>SNAMTQYTHIRNATGKLTIKNTTFLIDPFLAPKDTYPGFEGTFNYQQRMPMVDLPLSMDDLLSNVTAVVVTHTHLDHWDDTAINSIPKSLPIFVQNTADKELITSQGFIDVRIIFESLEFNGITLRKTGGSHGTVEMYANPVL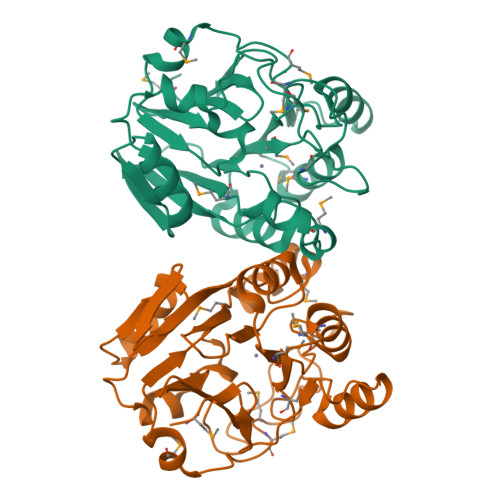APLAGDAMGVIFEAADEPTVYLVGDTVWTSDVEKALLRFDPNVIIMNTGYAQILGFEDSIIMGTKDIGRMVVRKPEAKIIAVHMDTVNHTATSRKDVRKFIKGNNIESHVAVPEDGETITL[4x]> GASNSYAIPENELLDEDTMNFISSLKNDLSNISNSLPFEYPHEIAEAIRSDFSNEDIYDNI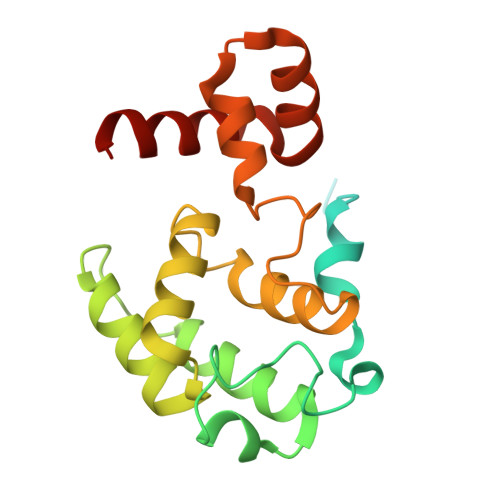DPDTISFPPKIATTDLFLPLFFHFGSTRQFMDKLHEVISGDYEPSQAEKLVQDLCDETGIRKNFSTSILTCLSGDLMVFPRYFLNMFKDNVNPPPNVPGIWTHDDDESLKSNDQEQIRKLVKKHGTGRMEMRKRFFEKDLL>[2x]MAHHHHHHVDDDDKMLTPAFDLSQDPDFLT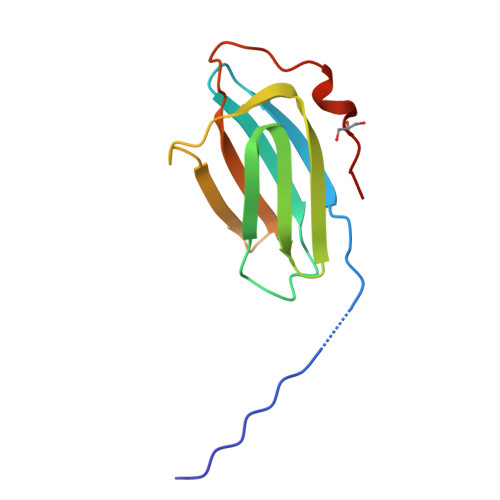IAIRVSYARVSEFDVYFEGSDFKFYAKPYFLRLTLPGRIVENGSEQGSYDADKGIFTIRLPKETPGQHFEGLNMLTALLA>[60x]MSENEIQDQQPSEPNDGQRGGGGGATGSVGGGKGSGVGISTGGWVGGSYFTDSYVITKNTRQFLVKIQNNHQYKTESIIPSNGGGKSQRCVSTPWSYFNFNQYSSHFSPQDWQRLTNEYKRFRPKGMHVKIYNLQIKQILSNGADVTYNNDLTAGVHIFCDGEHAYPNATHPWDEDVMPELPYQTWYLFQYGYIPTIHELAEMEDSNAVEKAIALQIPFFMLENSDHEVLRTGESAEFNFNFDCEWINNERAFIPPGLMFNPLVPTRRAQYIRRNGNTQASTSRVQPYAKPTSWMTGPGLLSAQRVGPAASDTAAWMVGVDPEGANINSGRAGVSSGFDPPAGSLRPTDLEYKVQWYQTPAGTNNDGNIISNPPLSMLRDQTLYRGNQTTYNLCSDVWMFPNQIWDRYPVTRENPIWCKQPRSDKHTTIDPFDGSIAMDHPPGTIF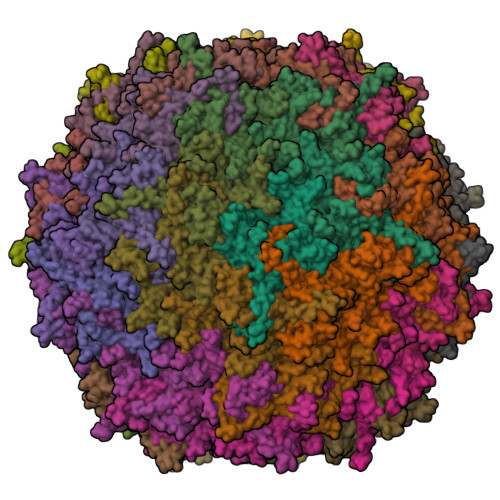IKMAKIPVPSNNNADSYLNIYCTGQVSCEIVWEVERYATKNWRPERRHTALGLGIGGADEINPTYHVDKNGAYIQPTTWDMCFPVKTNINKVL2-AMINO-4-[1-(CARBOXYMETHYL-CARBAMOYL)-2-(9-HYDROXY-7,8-DIOXO-7,8,9,10-TETRAHYDRO-BENZO[DEF]CHRYSEN-10-YLSULFANYL)-ETHYLCARBAMOYL]-BUTYRIC ACID | C30 H27 N3 O9 S | 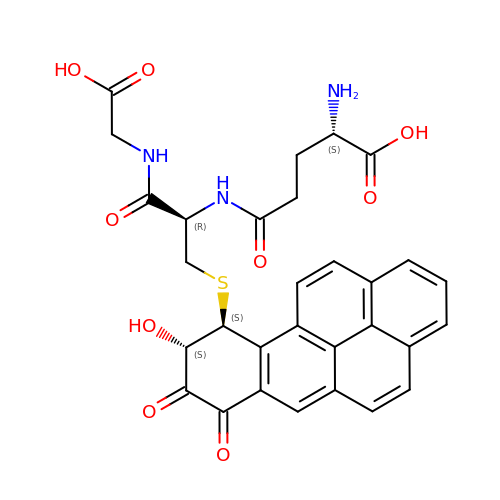DUWOHLGCRJLRRU-HVYZTVOGSA-N>[4x]MGSSHHHHHHSSENLYFQGHMNEIYQKAKHIKLFAMDVDGILSDGQIIYNSEGTETKA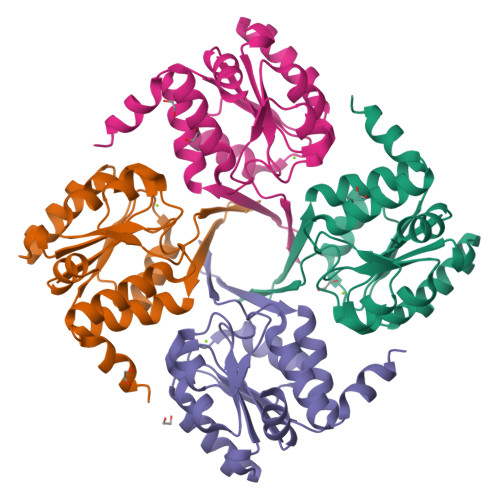FYVQDGLGLQALKQSGIILAIITGRSSAMVDRRAKELGISHIIQGQDDKLTALVGLTKKLGIELSHCAYIGDDLPDLKAVREAGFGISVPNGCEQTRAVSDYITTKTGGNGAVREVCELILKAQNNFDAFIATFQ> AMDLRVGRKFRIGRKIGSGSFGDIYHGTNLISGEEVAIRLESIRSRHPQLDYESRVYRYLSGGVGIPFIRWFGREGEYNAMVIDLLGPSLEDLFNYCHRRFSFKTVIMLALQMFCRIQYIHGRSFIHRDIKPDNFLMGVGRRGSTVHVIDFGLSKKYRDFNTHRHIPYRENKSLTGTARYASVNTHLGIEQSRRDDL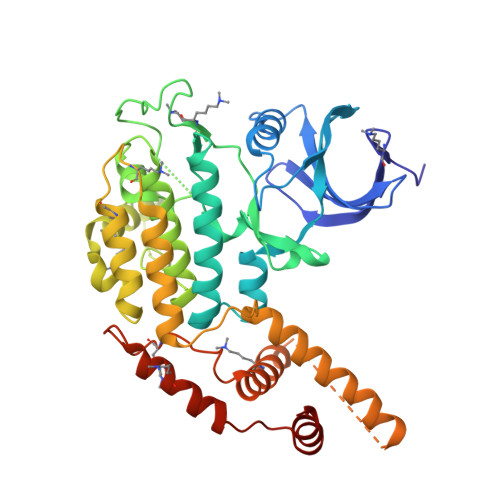ESLGYVLIYFCKGSLPWQGLKATTKKQKYDRIMEKKLNVSVETLCSGLPLEFQEYMAYCKNLKFDEKPDYLFLARLFKDLSIKLEYHNDHLFDWTMLRYTKAMVEKQRDLLIEKGDLNANSNAASASNSTDNKSETFNKIKLLAMKKFPTHFHYYKNEDKHNPSPEEIKQQTILNNNAASSLPEELLNALDKGMENLR>[4x]MTTELNQGEQFVADFRANAAALTTANAYNPEDEHDACGVGFIAAIDGKPRRSVVEKGIEALKAVWHRGAVDADGKTGDGAGIHVAVPQKFFKDHVKVIGHRAPDNKLAVGQVFLPRISLDAQEACRCIVETEILAFGYYIYGWRQVPINVDIIGEKANATRPEIEQIIVGNNKGVSDEQFELDLYIIRRRIEKAVKGEQINDFYICSLSARSIIYKGMFLAEQLTTFYPDLLDERFESDFAIYHQRYSTNTFPTWPLAQPFRMLAHNGEINTVKGNVNWMKAHETRMEHPAFGTHMQDLKPVIGVGLSDSGSLDTVFEVM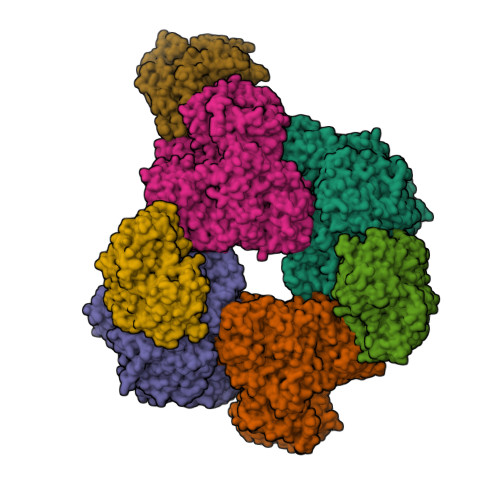VRAGRTAPMVKMMLVPQALTSSQTTPDNHKALIQYCNSVMEPWDGPAALAMTDGRWVVGGMDRNGLRPMRYTITTDGLIIGGSETGMVKIDETQVIEKGRLGPGEMIAVDLQSGKLYRDRELKDHLATLKPWDKWVQNTTHLDELVKTASLKGEPSDMDKAELRRRQQAFGLTMEDMELILHPMVEDGKEAIGSMGDDSPIAVLSDKYRGLHHFFRQNFSQVTNPPIDSLRERRVMSLKTRLGNLGNILDEDETQTRLLQLESPVLTTAEFRAMRDYMGDTAAEIDATFPVDGGPEALRDALRRIRQETEDAVRGGATHVILTDEAMGPARAAIPAILATGAVHTHLIRSNLRTFTSLNVRTAEGLDTHYFAVLIGVGATTVNAYLAQEAIAERHRRGLFGSMPLEKGMANYKKAIDDGLLKIMSKMGISVISSYRGGGNFEAIGLSRALVAEHFPAMVSRISGIGLNGIQKKVLEQHATAYNEEVVALPVGGFYRFRKSGDRHGWEGGVIHTLQQAVTNDSYTTFKKYSEQVNKRPPMQLRDLLELRSTKAPVPVDEVESITAIRKRFITPGMSMGALSPEAHGTLNVAMNRIGAKSDSGEGGEDPARFRPDKNGDNWNSAIKQVASGRFGVTAEYLNQCRELEIKVAQGAKPGEGGQLPGFKVTEMIARLRHSTPGVMLISPPPHHDIYSIEDLAQLIYDLKQINPDAKVTVKLVSRSGIGTIAAGVAKANADIILISGNSGGTGASPQTSIKFAGLPWEMGLSEVHQVLTLNRLRHRVRLRTDGGLKTGRDIVIAAMLGAEEFGIGTASLIAMGCIMVRQCHSNTCPVGVCVQDDKLRQKFVGTPEKVVNLFTFLAEEVREILAGLGFRSLNEVIGRTDLLHQVSRGAEHLDDLDLNPRLAQVDPGENARYCTLQGRNEVPDTLDARIVADARPLFEEGEKMQLAYNARNTQRAIGTRLSSMVTRKFGMFGLQPGHITIRLRGTAGQSLGAFAVQGIKLEVMGDANDYVGKGLSGGTIVVRPTTSSPLETNKNTIIGNTVLYGATAGKLFAAGQAGERFAVRNSGATVVVEGCGSNGCEYMTGGTAVILGRVGDNFAAGMTGGMAYVYDLDDSLPLYINDESVIFQRIEVGHYESQLKHLIEEHVTETQSRFAAEILNDWAREVTKFWQVVPKEMLNRLEVPVHLPKAISAE;>MANQRMLGFVHTAQRMPDKRPAAERRQDFAEIYARFSDERANEQANRCSQCGVPFCQVHCPVSNNIPDWLKLTSEGRLEEAYEVSQATNNFPEICGRICPQDRLCEGNCVIEQSTHGAVTIGSVEKYINDTAWDQGWVKPRTPSRELGLSVGVIGAGPAGLAAAEELRAKGYEVHVYDRYDRMGGLLVYGIPGFKLEKSVVERRVKLLADAGVIYHPNFEVGRDASLPELRRKHVAVLVATGVYKARDIKAPGSGLGNIVAALDYLTTSNKVSLGDTVEAYENGSLNAAGKHVVVLGGGDTAMDCVRTAIRQGATSVKCLYRRDRKNMPGSQREVAHAEEEGVEFIWQAAPEGFTGDTVVTGVRAVRIHLGVADATGRQTPQVIEGSEFTVQADLVIKALGFEPEDLPNAFDEPELKVTRWGTLLVDHRTKMTNMDGVFAAGDIVRGASLVVWAIRDGRDAAEGIHAYAKAKAEAPVAVAAE[3x]>[2x]RKTNTTATEVA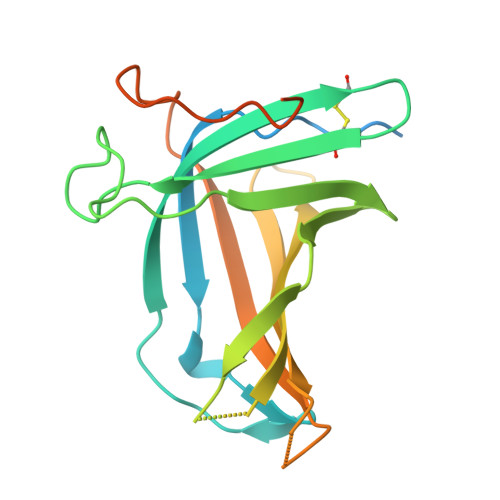RPPTSGSAVPSAPTTTVAVTAPVPLDGTYRIEIQRSKQTYDYTPTPQPPDVNTWWAFRTSCTPTECLAAATMLDDNDHTQAKTPPVRPFLMQFGEGQWKSRPETVQFPCVGPNGSPSTQATTQLLALRPQPQGDLVGEMVVTVHSNECGQQGAVIRIPAVASRSGDLPPAVTVPDPATIPDTPDTTSTATLTPPTTTAPGPGR>[7x]GPGMKINTTGGQIHGITQDGLD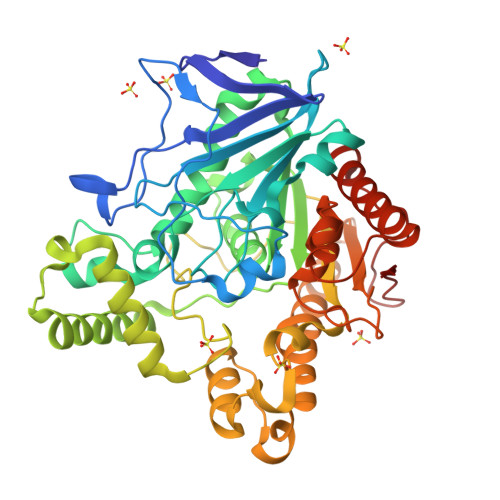IFLGIPYAEPPVHDNRFKHSTLKTQWSEPIDATEIQPIPPQPDNKLEDFFSSQSTTFTEHEDCLYLNIWKQHNDQTKKPVIIYFYGGSFENGHGTAELYQPAHLVQNNDIIVITCNYRLGALGYLDWSYFNKDFHSNNGLSDQINVIKWVHQFIESFGGDANNITLMGQSAGSMSILTLLKIPDIEPYFHKVVLLSGALRLDTLESARNKAQHFQKMMLDYLDTDDVTSLSTNDILMLMAKLKQSRGPSKGLDLIYAPIKTDYIQNNYPTTKPIFACYTKDEGDIYITSEQKKLSPQRFIDIMELNDIPLKYEDVQTAKQQSLAITHCYFKQPMKQFLQQLNIQDSNAQLWLAEFAWHDTSSAHYRSAYHILDMVFWFGNLQILAAHQYPTTAHLKFLSRQMQNDLANFAKSGKMPWPMYHNERRYYRTYQ8-AMINOGUANINE | C5 H6 N6 O | 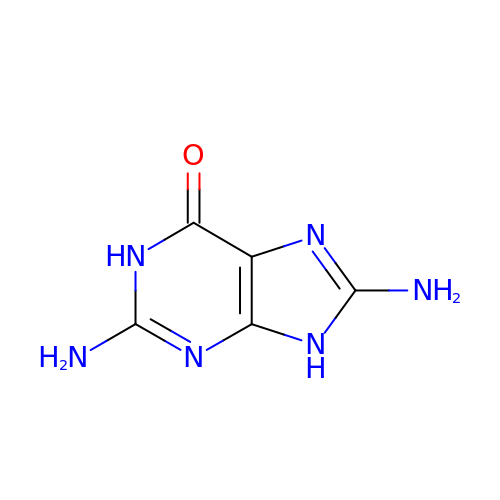WYDKPTZGVLTYPG-UHFFFAOYSA-N Phosphoglycerate kinase 1 (PGK1) is an ubiquitous enzyme expressed in all somatic cells that plays a central role in glycolysis where it provides energy in form of ATP through the reversible phosphotransfer reaction from 1,3-bisphosphoglycerate (1,3-BPG) to MgADP in order to produce 3-phosphoglycerate (3-PG) and MgATP in the presence of free magnesium. PGK1 is a monomeric enzyme of 417 amino acids formed by two distinct α-helical domains of equal size, the N- and C-terminal domains connected by a hinge region. The N-terminal domain binds 3-PG or 1,3-BPG while the C-terminal domain binds MgADP or MgATP. Two different crystallographic conformations of PGK1 have been already identified: the partially closed conformation, able to bind substrates, and the closed conformation, the catalytically competent state.

V216 belongs to the loop 214–219, close to the ADP-binding site. The rearrangement of this loop has been suggested to be important for the enzyme transition to the closed conformation upon binding of the two ligands. Indeed, in the wild type structure in complex with the MgADP ligand the loop assumes two conformations, promoting the reorientation of K215 and D218, now ready to interact with γ-phosphate of 3-PG and D65, in the closed conformation. In the V216F variant structure in complex with MgADP, the loop adopts the same conformation as in apo-PGK1. Replacement of the valine with a phenylalanine keeps the loop in the apo-like conformation since the aromatic residue tends to stay buried. The lower mobility of the loop hampers the transition from the open to the closed conformation affecting the enzyme catalytic activity (the kcat of the mutant is 1.9 s-1, 45-fold lower than that of the wild type). Conversely, no variation is found in ADP-binding. In fact, as shown in Fig 5, the residues directly involved in the ADP binding (E343, G312, A214) and the Mg2+ion bound through the β and γ-phosphate and D374 preserve the same positions as in the wild type structure. In this variant, the introduction of a phenylalanine residue reinforces the hydrophobic interactions between the 211–219 loop and the 243–263 region thereby stabilizing the C-terminal domain. This local stabilization, which decreases the flexibility of the ATP binding site, is sufficient to determine the decrease of about 50-fold of the turnover number with respect to that of the wild type protein.

> SLSNKLTLDKLDVKGKRVVMRVDFNVPMKNNQITNNQRIKAAVPSIKFCLDNGAKSVVLMSHLGRPDGVPMPDKYSLEPVAVELKSLLGKDVLFLKDCVGPEVEKACANPAAGSVILLENLRFHVEEEGKGKDASGNKVKAEPAKIEAFRASLSKLGDVYVNDAFGTAHRAHSSMVGVNLPQKAGGFLMKKELNYFAKALESPERPFLAILGGAKFADKIQLINNMLDKVNEMIIGGGMAFTFLKVLNNMEIGTSLFDEEGAKIVKDLMSKAEKNGVKITLPVDFVTADKFDENAKTGQATVASGIPAGWMGLDCGPESSKKYAEAVTRAKQIVWNGPVGVFEWEAFARGTKALMDEVVKATSRGCITIIGGGDTATCCAKWNTEDKVSHVSTGGGASLELLEGKVLPGVDALSNI>[4x]SLMNKSQQVQTITLAAAQQMAAAVEKKATEINVAVVFSVVDRGGNTLLIQRMDE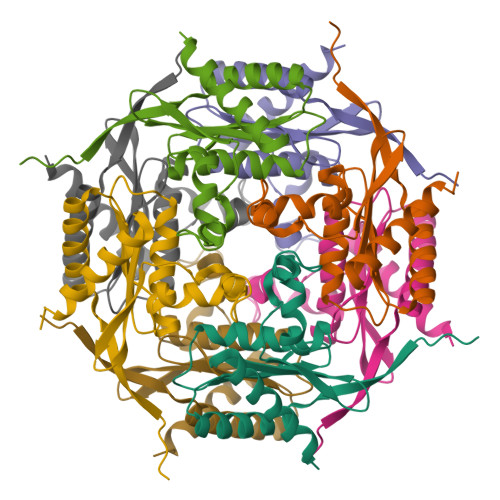AFVSSCDISLNKAWSACSLKQGTHEITSAVQPGQSLYGLQLTNQQRIIIFGGGLPVIFNEQVIGAVGVSGGTVEQDQLLAQCALDCFSALE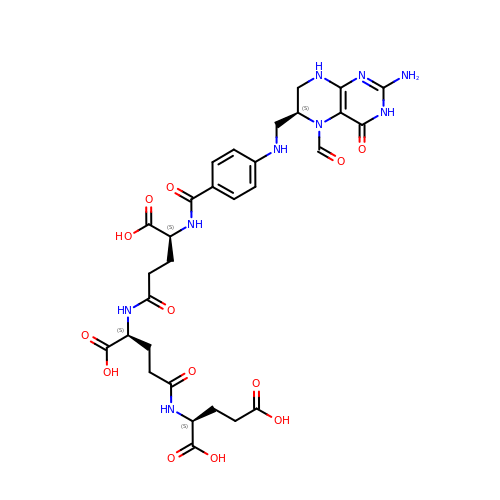2-[4-(4-{4-[(2-AMINO-5-FORMYL-4-OXO-3,4,5,6,7,8-HEXAHYDRO-PTERIDIN-6-YLMETHYL)-AMINO]-BENZOYLAMINO}-4-CARBOXY-BUTYRYLAMINO)-4-CARBOXY-BUTYRYLAMINO]-PENTANEDIOIC ACID | C30 H37 N9 O13 | ZLOMJLIQXBKNHU-VJANTYMQSA-N1,7-di-O-phosphono-beta-D-altro-hept-2-ulofuranose | C7 H16 O13 P2 | 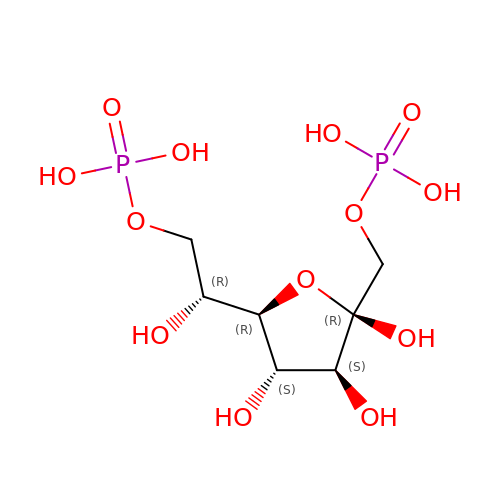YCQNLCZEHKXXNQ-BNWJMWRWSA-N>[2x]MTLVLRYAARSDRGLVRANNEDSVYAGARLLALADGMGGHAAGEVASQLVIAALAHLDDDEPGGDLLAKL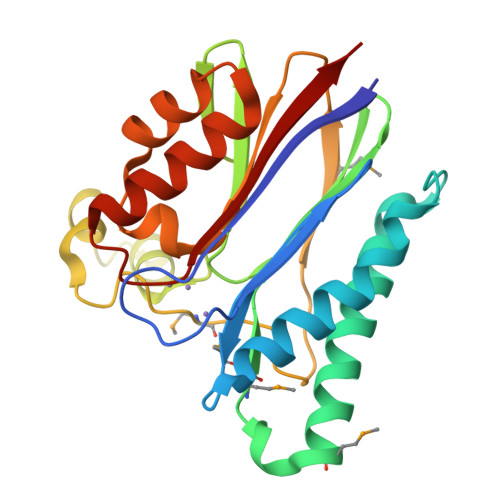DAAVRAGNSAIAAQVEMEPDLEGMGTTLTAILFAGNRLGLVHIGDSRGYLLRDGELTQITKDDTFVQTLVDEGRITPEEAHSHPQRSLIMRALTGHEVEPTLTMREARAGDRYLLCSDGLSDPVSDETILEALQIPEVAESAHRLIELALRGGGPDNVTVVVADLEH Among human species B adenovirus, HAdV-11, has the particular feature of exploiting two primary receptors, desmoglein 2 (DSG2) and CD46, to mediate cell attachment. Interactions between HAdV-11 and CD46 are well-characterized and clearly depend on the fiber protein, but the mechanism whereby HAdV-11 engages DSG2 has been still unresolved. In this study, we elucidate the molecular basis for HAdV-11 recognition of DSG2 by resolving the structure of extracellular domains of DSG2 in complex with the HAdV-11 fiber knob protein. The structure shows that DSG2 and CD46 engage different HAdV-11 residues and interfaces without overlapping.

Based on the successful strategy of our previous work, the structure of HAd11K/ rDSG2 was solved by cryoEM. During the image analysis, two main populations of particles consisting of the HAd11K in complex with either one or two rDSG2 modules were identified and two 3D reconstructions were obtained at 3.5 and 3.2 Å resolution for HAd11K in complex with one or two rDSG2, respectively. The binding of rDSG2 to HAd11K is very similar in both populations meaning that the binding of a second rDSG2 is possible without interfering with the first rDSG2. The tips of two loops in EC2 (around residue A125 and residues S175, T177, respectively) are in close contact with residues located on the apex of the HAd11K (in particular residues N190 and N192). Several putative hydrogen bonds are predicted in this region which likely contributes to the binding. Regarding the interaction of the EC3 module of rDSG2 with HAd11K, the loop region centered around R316 of EC3 fits snugly in an apical region of HAd11K defined by two loops centered around D265 and D300, respectively. Several hydrogen bonds and salt bridges are also predicted in this area. As reported for the other two serotypes, −3 and −7, the structure shows that EC2 and EC3 ectodomains bind at the top of the trimeric knob and that D265 mediates central contacts with DSG2 (19, 21). Interestingly, the critical D265 residue interacting with the EC3 domain of DSG2 is also seen in HAd11K confirming the importance of this pocket for all DSG2-interacting serotypes. We, therefore, produced a D265A mutant of HAd11K and subjected to BLI experiments, clearly indicated that D265 is, indeed, a key residue for stabilizing the complex with DSG2.

>MTKRVRLSDSFNPVYPYEDESTSQHPFINPGFISPNGFTQSPNGVLTLKCLTPLTTTGGSLQLKVGGGLTVDDTNGFLKENISATTPLVKTGHSIGLPLGAGLGTNENKLCIKLGQGLTFNSNNICIDDNINTLWTGVNPTEANCQIMNSSESNDCKLILTLVKTGALVTAFVYVIGVSNNFNMLTTHRNINFTAELFFDSTGNLLTRLSSLKTPLNHKSGQNMATGAITNAKGFMPSTTAYPFNDNSREKENYIYGTCYYTASDRTAFPIDISVMLNRRAINDETSYCIRITWSWNTGDAPEVQTSATTLVTSPFTFYYIREDD[3x];> MARSPGRAYALLLLLICFNVGSGLHLQVLSTRNENKLLPKHPHLVRQKRAWITAPVALREGEDLSKKNPIAKIHSDLAEERGLKITYKYTGKGITEPPFGIFVFNKDTGELNVTSILDREETPFFLLTGYALDARGNNVEKPLELRIKVLDINDNEPVFTQDVFVGSVEELSAAHTLVMKINATDADEPNTLNSKISYRIVSLEPAYPPVFYLNKDTGEIYTTSVTLDREEHSSYTLTVEARDGNGEVTDKPVKQAQVQIRILDVNDNIPVVENKVLEGMVEENQVNVEVTRIKVFDADEIGSDNWLANFTFASGNEGGYFHIETDAQTNEGIVTLIKEVDYEEMKNLDFSVIVANKAAFHKSIRSKYKPTPIPIKVKVKNVKEGIHFKSSVISIYVSESMDRSSKGQIIGNFQAFDEDTGLPAHARYVKLEDRDNWISVDSVTSEIKLAKLPDFESRYVQNGTYTVKIVAISEDYPRKTITGTVLINVEDINDNCPTLIEPVQTICHDAEYVNVTAEDLDGHPNSGPFSFSVIDKPPGMAEKWKIARQESTSVLLQQSEKKLGRSEIQFLISDNQGFSCPEKQVLTLTVCECLHGSGCREAQHDSYVGLGPAAIALMILAFLLLLLVPLLLLMCHCGKGAKGFTPIPGTIEMLHPWNNEGAPPEDKVVPSFLPVDQGGSLVGRNGVGGMAKEATMKGSSSASIVKGQHEMSEMDGRWEEHRSLLSGRATQFTGATGAIMTTETTKTARATGASRDMAGAQAAAVALNEEFLRNYFTDKAASYTEEDENHTAKDCLLVYSQEETESLNASIGCCSFIEGELDDRFLDDLGLKFKTLAEVCLGQKIDINKEIEQRQKPATETSMNTASHSLCEQTMVNSENTYSSGSSFPVPKSLQEANAEKVTQEIVTERSVSSRQAQKVATPLPDPMASRNVIATETSYVTGSTMPPTTVILGPSQPQSLIVTERVYAPASTLVDQPYANEGTVVVTERVIQPHGGGSNPLEGTQHLQDVPYVMVRERESFLAPSSGVQPTLAMPNIAVGQNVTVTERVLAPASTLQSSYQIPTENSMTARNTTVSGAGVPGPLPDFGLEESGHSNSTITTSSTRVTKHSTVQHSYS>[4x]MEGPLTIPVLDKGFVRLVDQMGDDRAIVQAARVSYGEGTKTVREDAALIDYLMRHRHTSPFEMVVFKFHVKAPIFVARQWFRHRTASVNEISGRYSILKEEFYEPEAFRKQA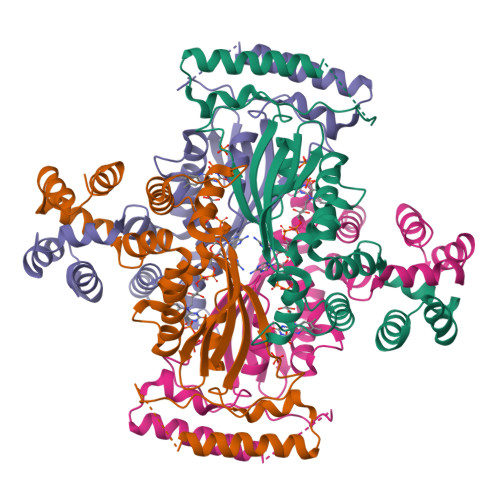KRNKQASEGALLDEEALALLRKVQQEAYGAYRALLEKGVAREMARMVLPLNLYTEFYWKQDLHNLFHFLKLRLAPEAQWEIRQYARAIAEIVKERVPLAWAAFEEHLLEGAFLSRTELRALRGLLTPEVYEKALSSLGLGGSRLKEALEKVFGPGEAL> MGRRRSHERRDLPPNLYIRNNGYYCYRDPRTGKEFGLGRDRRIAITEAIQANIELFSGHKHKPLTARINSDNSVTLHSWLDRYEKILASRGIKQKTLINYMSKIKAIRRGLPDAPLEDITTKEIAAMLNGYIDEGKAASAKLIRSTLSDAFREAIAEGHITTNHVAATRAAKSEVRRSRLTADEYLKIYQAAESSPCWLRLAMELAVVTGQRVGDLCEMKWSDIVDGYLYVEQSKTGVKIAIPTALHIDALGISMKETLDKCKEILGGETIIASTRREPLSSGTVSRYFMRARKASGLSFEGDPPTFHELRSLSARLY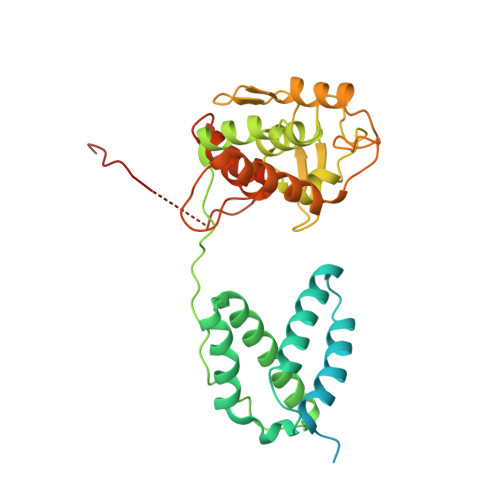EKQISDKFAQHLLGHKSDTMASQYRDDRGREWDKIEIK>[8x]PYEWENPQLVSEGTEKSHASFIPYLDPFSGEWEYPEEFISLNGNWRFLFAKNPFEVPEDFFSEKFDDSNWDEIEVPSNWEMKGYGKPIYTNVVYPFEPNPPFVPKDDNPTGVYRRWIEIPEDWFKKEIFLHFEGVRSFFYLWVNGKKIGFSKDSCTPAEFRLTDVLRPGKNLITVEVLKWSDGSYLEDQDMWWFAGIYRDVYLYALPKFHIRDVFVRTDLDENYRNGKIFLDVEMRNLGEEEEKDLEVTLITPDGDEKTLVKETVKPEDRVLSFAFDVKDPKKWSAETPHLYVLKLKLGEDEKKVNFGFRKIEIKDGTLLFNGKPLYIKGVNRHEFDPDRGHAVTVERMIQDIKLMKQHNINTVRTSHYPNQTKWYDLCDYFGLYVIDEANIESHGIDWDPEVTLANRWEWEKAHFDRIKRMVERDKNHPSIIFWSL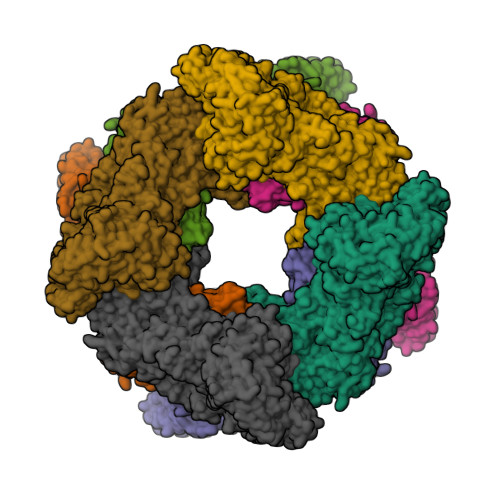GNEAGDGVNFEKAALWIKKRDNTRLIHYEGTTRRGESYYVDVFSLMYPKMDILLEYASKKREKPFIMCEYAHAMGNSVGNLKDYWDVIEKYPYLHGGCIWDWVDQGIRKKDENGREFWAYGGDFGDTPNDGNFCINGVVLPDRTPEPELYEVKKVYQNVKIRQVSKDTYEVENRYLFTNLEMFDGAWKIRKDGEVIEEKTFKIFAEPGEKRLLKIPLPEMDDSEYFLEISFSLSEDTPWAEKGHVVAWEQFLLKAPAFEKKSISDGVSLREDGKHLTVEAKDTVYVFSKLTGLLEQILHRRKKILKSPVVPNFWRVPTDNDIGNRMPQRLAIWKRASKERKLFKMHWKKEENRVSVHSVFQLPGNSWVYTTYTVFGNGDVLVDLSLIPAEDVPEIPRIGFQFTVPEEFGTVEWYGRGPHETYWDRKESGLFARYRKAVGEMMHRYVRPQETGNRSDVRWFALSDGETKLFVSGMPQIDFSVWPFSMEDLERVQHISELPERDFVTVNVDFRQMGLGGDDSWGAMPHLEYRLLPKPYRFSFRMRISEEIPSWRVLAAIPETLHVEMSSEDVIREGDTLRVKFSLLNDTPLSKEKQVVLFVDGNEYSVRRVVIPPFKKEELVFKVEGLKKGEHLIHTNLNTRKTIYVR> GPLGSMTTDEGAKNNEESPTATVAEQGEDITSKKDRGVLKIVKRVGNGEETPMIGDKVYVHYKGKLSNGKKFDSSHDRNEPFVFSLGKGQVIKAWDIGVATMKKGEICHLLCKPEYAYGSAGSLPKIPSNATLFFEIELLDFKGEDLFEDGGIIRRTKRKGEGYSNPNEGATVEIHLEGRCGGRMFDCRDVAFTVGEGEDHDIPIGIDKALEKMQREEQCILYLGPRYGFGEAGKPKFGIEPNAELIYEVTLKSFEKAKESWEMDTKEKLEQ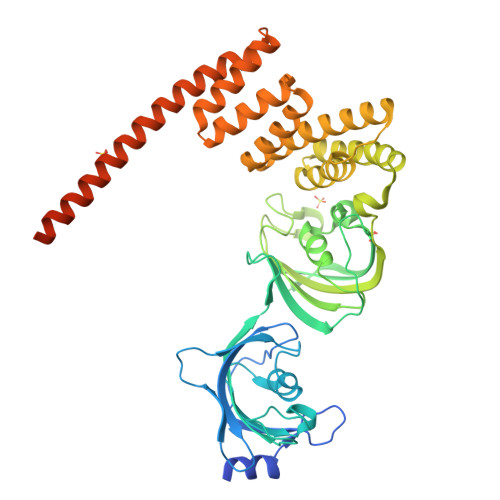AAIVKEKGTVYFKGGKYMQAVIQYGKIVSWLEMEYGLSEKESKASESFLLAAFLNLAMCYLKLREYTKAVECCDKALGLDSANEKGLYRRGEAQLLMNEFESAKGDFEKVLEVNPQNKAARLQISMCQKKAKEHNERDRRIYANMFKKFAEQDAKEEANKAMGKKTSEGVTNEKGTDSQAMEEEKPEGHV> MDFDMIEEKKDSVIVRNVENFELKDIFDCGQCFRWHRQENGNYIGIAFEKVVEVQKIGEDVVIYNINEEEFKNVWSEYFDLYRDYGEIKKELSRDPLLKKSVDFGEGIRILRQDPFEILLSFIISANNRIPMIKKCINNISEKAGKKLEYKGKIYYAFPTVDKLHEFTEKDFEECTAGFRAKYLK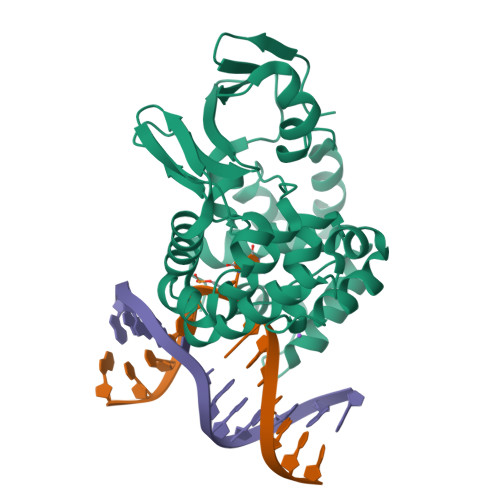DTVDRIYNGELNLEYIKSLNDNECHEELKKFMGVGPQVADCIMLFSMQKYSAFPVDTWVKKAMMSLYVAPDVSLKKIRDFGREKFGSLSGFAQQYLFYYARENNIQ> MEMDIRFRGDDPEAYYKALREMIRQARKFAGTVTVTLIIRFRGDDLEALEKALKEMIRQARKFAGTVTYTLDGNDLEIRITGV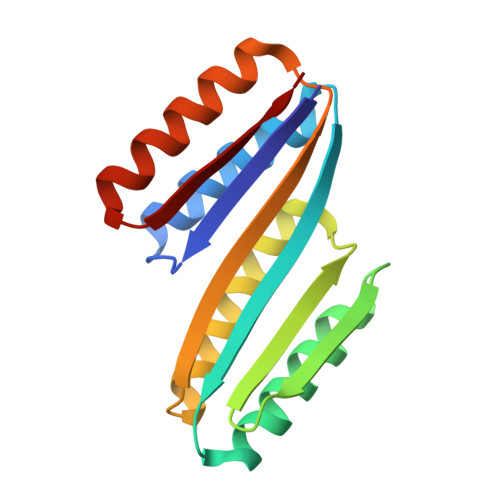PPQVILELVKEAIRLAKEFNITVTVELVIRITGVPEQVRKELAKEAERLAKEFNITVTYTIRL>[2x]GMQTTEIDLRL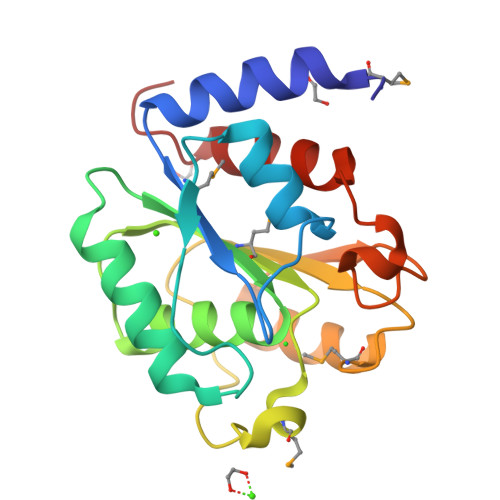TEVSQQLTMVLVPGLRDSDDEHWQSHWERRFPHWQRIRQREWYQADLDRWVLAIRRELSVCTQPVILIGHSFGALAACHVVQQGQEGIAGVMLVAPAEPMRFEIDDRIQASPLSVPTLTFASHNDPLMSFTRAQYWAQAWDSELVDVGEAGHINAEAGFGPWEYGLKRLAEFSEILIPNR> GPHMAH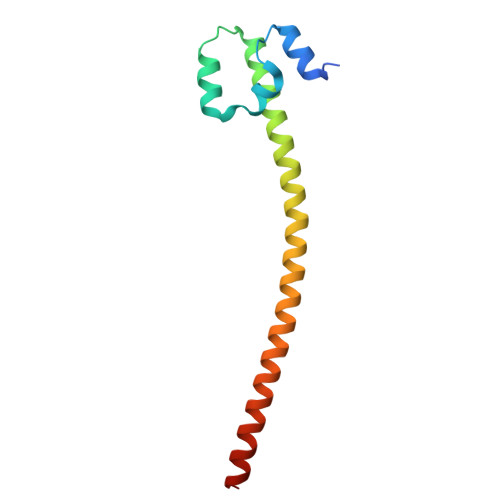LTRDELRAKALHIPFPVEKIINLPVVDFNEMMSKEQFNEAQLALIRDIRRRGKNKVAAQNCRKRKLENIVELEQDLDHLKDEKEKLLKEKGENDKSLHLLKKQLSTL> MFTRRGDQGETDLANRARVGKDSPVVEVQGTIDELNSFI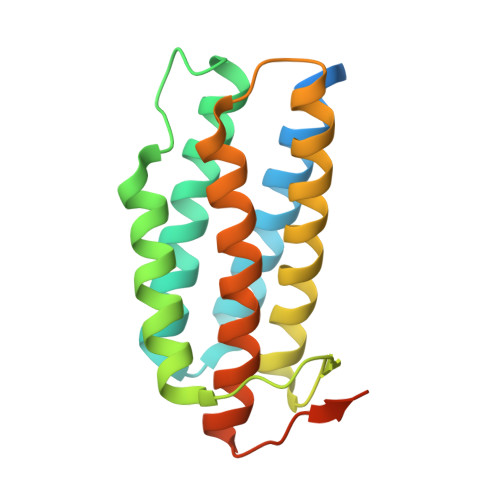GYALVLSRWDDIRNDLFRIQNDLFVLGEDVSTGGKGRTVTMDMIIYLIKRSVEMKAEIGKIELFVVPGGSVESASLHMARAVSRRLERRIKAASELTEINANVLLYANMLSNILFMHALISNKRLNIPEKIWSIHRVSLEHHHHHH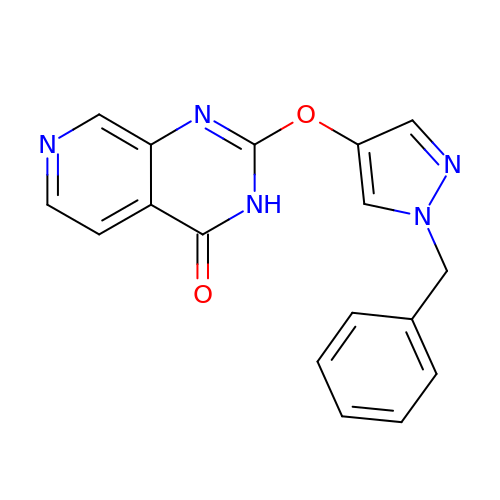2-[(1-benzyl-1H-pyrazol-4-yl)oxy]pyrido[3,4-d]pyrimidin-4(3H)-one | C17 H13 N5 O2 | ZTYRLXUTLYBVHH-UHFFFAOYSA-N> ASAECVSNENVEIEAPKTNIWTSLAKEEVQEVLDLLHSTYNITEVTKADFFSNYVLWIETLKPNKTEALTYLDEDGDLPPRNARTVVYFGEGEEGYFEELKVGPLPVSDETTIEPLSFYNTNGKSKLPFEVGHLDRIKSAAKSSFLNKNLNTTIMRDVLEGLIGVPYEDMGCHSAAPQLHDPATGATVDYGTCNINTENDAENLVPTGFFFKFDMTGRDVSQWKMLEYIYNNKVYTSAEELYEAMQKDDFVTLPKIDVDNLDWTVIQRNDSAPVRHLDDRKSPRLVEPEGRRWAYDGDEEYFSWMDWGFYTSWSRDTGISFYDITFKGERIVYELSLQELIAEYGSDDPFNQHTFYSDISYGVGNRFSLVPGYDCPSTAGYFTTDTFEYDEFYNRTLSYCVFENQEDYSLLRHTGASYSAITQNPTLNVRFISTIGNYDYNFLYKFFLDGTLEVSVRAAGYIQAGYWNPETSAPYGLKIHDVLSGSFHDHVLNYKVDLDVGGTKNRASQYVMKDVDVEYPWAPGTVYNTKQIAREVFENEDFNGINWPENGQGILLIESAEETNSFGNPRAYNIMPGGGGVHRIVKNSRSGPETQNWARSNLFL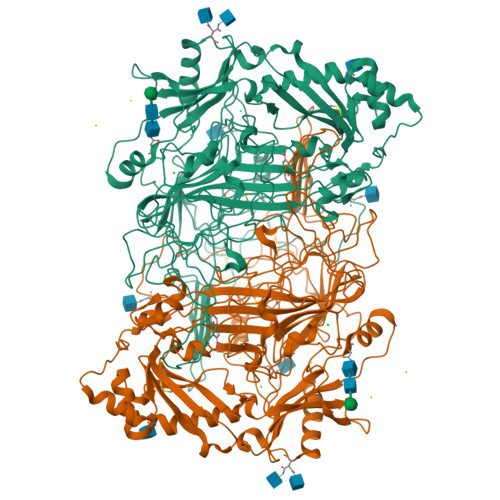TKHKDTELRSSTALNTNALYDPPVNFNAFLDDESLDGEDIVAWVNLGLHHLPNSNDLPNTIFSTAHASFMLTPFNYFDSENSRDTTQQVFYTYDDETEESNWEFYGNDWSSCGVEVAEPNFEDYTYGRGTRINKKMTNSDEVY>MSSTILVIHGPNLNLLGKREPEVYGHLTLDNINRQL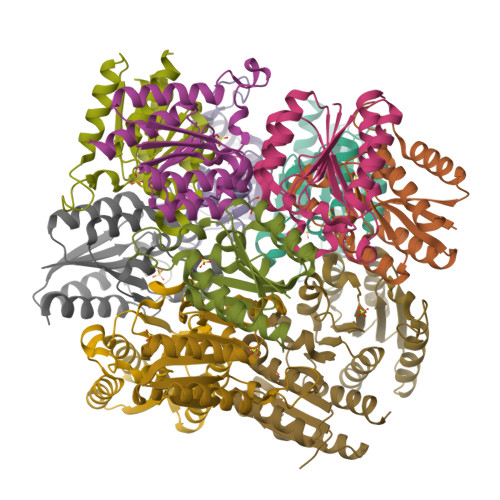IAQAEQASITLDTFQSNWEGAIVDRIHQAQTEGVKLIIINPAALTHTSVALRDALLGVAIPFIEVHLSNVHAREAFRHHSYLSDKAIGVICGLGAKGYSFALDYAIEKIQPSNPN[12x]>GNGKLRQWLIDQIDSGKYPGLVWENEEKSIFRIPWKHAGKQDYNREEDAALFKAWALFKGKFREGIDKPDPPTWKRRLR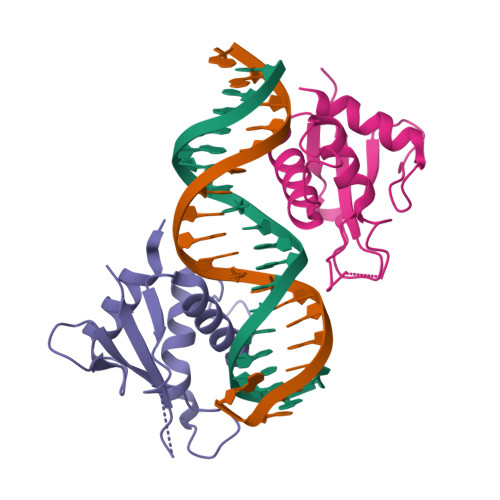CALNKSNDFEELVERSQLDISDPYKVYRIVPEGAKKG[4x]> MVMGIFANCIFCLKVKYLPQQQKKKLQTDIKENGGKFSQSLNPQCTHIILDNADVLSQYQLNSIQKNHVHIANPDFIWKSIREKRLLDVKNYDPYKPLDI

pmcPARP4 is an ADP-ribosyltransferase (ART) that uses NAD+ as substrate to add ADP-ribose onto target proteins, a process called mono(ADP-ribosylation) or MARylation. PARP4 is also referred to as vault PARP since it can localize to the vault particle, a cytoplasmic ribonucleoprotein complex. PARP4 has a distinct domain composition relative to other PARP enzymes; however, the N-terminal region of PARP4 is homologous to a collection of domains found in PARP1, a regulator of multiple nuclear processes including the cellular response to DNA damage. Collectively, the study establishes the human PARP4 BRCT as a nucleic acid–binding module.

However, the location of Phe39 on the potential nucleic acid–binding surface was intriguing so we also considered Phe39 as a possibly important residue. Conservation analysis using ConSurf indicated that Phe39 is conserved in 77% of 150 PARP4 homologs. We mutated Phe39 to glutamine and to alanine to test the importance of this region. We determined X-ray structures of the four PARP4 BRCT domain mutants. As expected from thermal stability analysis, the overall BRCT fold was not affected by the different mutations, and superposition of the mutant structures with WT BRCT yielded RMSD values between 0.5 and 0.8 Å (comparing all 763–788 atoms). Mutants F39A and F39Q both led to a shift in the position of the sidechain of K23, which impacted the charge distribution at the structure surface beyond just the F39 location. The loop that bears residue F39 was repositioned in the F39Q mutant, whereas this loop did not change in the F39A mutant, thus leading to visible changes in the electrostatic surface potential. Relative to WT BRCT (0.5 ± 0.2 μM), mutants F39Q and F39A exhibited slightly weakened binding, with estimated KD values of 0.9 ± 0.5 μM and 0.6 ± 0.1 μM, respectively. Relative to WT BRCT (KD of 19 ± 4 μM), F39Q and F39A showed weakened binding with KD values of 35 ± 10 μM and 33 ± 2 μM, respectively. The TM of WT BRCT was measured as 51.6 °C ± 0.2 deg, whereas TM values of 54.7 °C ± 0.4 deg, 54.3 °C ± 1 deg, 58 °C ± 1 deg, and 60.0 °C ± 0.7 deg were obtained for BRCT mutants F39A, F39Q, K31Q, and K23/24Q, respectively.>[2x]MVPISPIETVPVKLKPGMDGPKVKQWPLTEEKIKALVEICTEMEKEGKISKIGPENPYNTPVFAIKKKDSTKWRKLVDFRELNKRTQDFWEVQLGIPHPAGLKKKKSVTVLDVGDAYFSVPLDEDFRKYTAFTIPSINNETPGIRYQYNVLPQGWKGSPAIFQSSMTKILEPFKKQNPDIVIYQYMDDLYVGSDLEIGQHRTKIEELRQHLLRWGLTTPDKKHQKEPPFLWMGYELHPDKWTVQPIVLPEKDSWTVNDIQKLVGKLNWASQIYPGIKVRQLCKLLRGTKALTEVIPL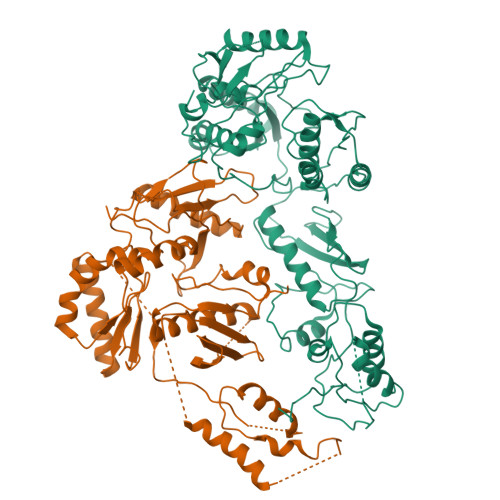TEEAELELAENREILKEPVHGVYYDPSKDLIAEIQKQGQGQWTYQIYQEPFKNLKTGKYARMRGAHTNDVKQLTEAVQKITTESIVIWGKTPKFKLPIQKETWETWWTEYWQATWIPEWEFVNTPPLVKLWYQLEKEPIVGAETFYVDGAANRETKLGKAGYVTNKGRQKVVPLTNTTNQKTELQAIYLALQDSGLEVNIVTDSQYALGIIQAQPDKSESELVNQIIEQLIKKEKVYLAWVPAHKGIGGNEQVDKLVSAGENLYFQ>[4x]MNLLRRSGKRRRSESGSDSFSGSGGDSSASPQFLSGSVLSPPPGLGRCLKAAAAGECKPTVPDYERDKLLLAN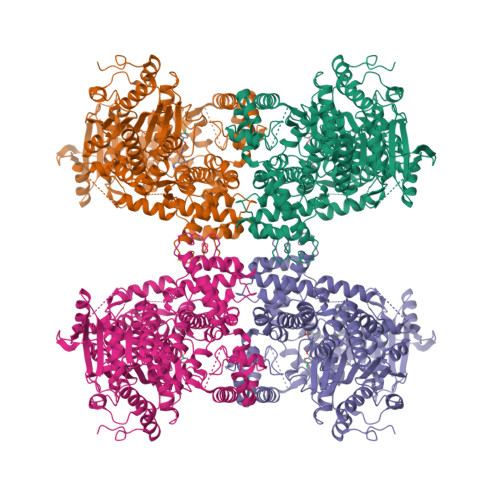WGLPKAVLEKYHSFGVKKMFEWQAECLLLGQVLEGKNLVYSAPTSAGKTLVAELLILKRVLEMRKKALFILPFVSVAKEKKYYLQSLFQEVGIKVDGYMGSTSPSRHFSSLDIAVCTIERANGLINRLIEENKMDLLGMVVVDELHMLGDSHRGYLLELLLTKICYITRKSASCQADLASSLSNAVQIVGMSATLPNLELVASWLNAELYHTDFRPVPLLESVKVGNSIYDSSMKLVREFEPMLQVKGDEDHVVSLCYETICDNHSVLLFCPSKKWCEKLADIIAREFYNLHHQAEGLVKPSECPPVILEQKELLEVMDQLRRLPSGLDSVLQKTVPWGVAFHHAGLTFEERDIIEGAFRQGLIRVLAATSTLSSGVNLPARRVIIRTPIFGGRPLDILTYKQMVGRAGRKGVDTVGESILICKNSEKSKGIALLQGSLKPVRSCLQRREGEEVTGSMIRAILEIIVGGVASTSQDMHTYAACTFLAASMKEGKQGIQRNQESVQLGAIEACVMWLLENEFIQSTEASDGTEGKVYHPTHLGSATLSSSLSPADTLDIFADLQRAMKGFVLENDLHILYLVTPMFEDWTTIDWYRFFCLWEKLPTSMKRVAELVGVEEGFLARCVKGKVVARTERQHRQMAIHKRFFTSLVLLDLISEVPLREINQKYGCNRGQIQSLQQSAAVYAGMITVFSNRLGWHNMELLLSQFQKRLTFGIQRELCDLVRVSLLNAQRARVLYASGFHTVADLARANIVEVEVILKNAVPFKSARKAVDEEEEAVEERRNMRTIWVTGRKGLTEREAAALIVEEARMILQQDLVEM>MSLKTNFVKYERKDNKDLCEITLENDAGMAVKVLNYGATLEKVLLDGENMILSLNSPEDYSKERNFLGGTVGRIAGRVRAGQWKHGNEIHQLPLNDGDNHIHGGIGTDMHVWDFRPSCDSEHARVDLTLFDPDGNNDYPGNLKLHARYELDNENNLHYLLEAVSDKLTIFNPVNHTYFNLGERAEDLNLQMNADYYLPVDEAGLPDRGMAEVAGTAFDFRKTKRIGDALNSDDSQIKLRNGLDHPFILNGNNPAALLSSNKHRLIVKTNAPALVLYAGNHFNHTGIVNNIGQYDGITFEAQCPPAEGNDLGQITLLPFEKFKRT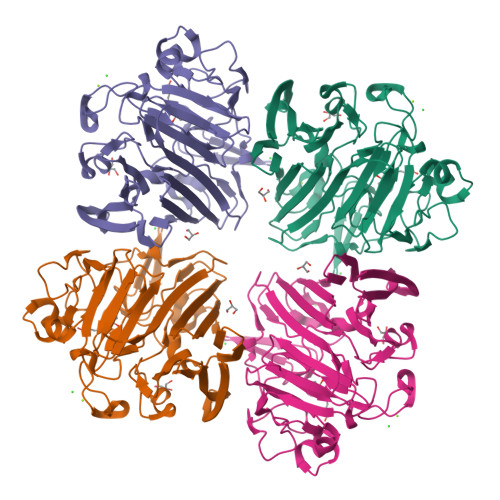VDWKFEEGHHHHHH[2x]> MSLESMLSHPPIPIADMAEHTERLKANDSLKLSQEYESIDPGQQFTWEHSNLEVNKPKNRYANVIAYDHSRVILQPIEGIMGSDYINANYVDGYRRQNAYIATQGPLPETFGDFWRMVWEQRSATIVMMTRLEEKSRIKCDQYWPNRGTETYGFIQVTLLDTIELATFCVRTFSLHKNGSSEKREVRQFQFTAWPDHGVPEYPTPFLAFLRRVKTCNPPDAGPIVVHCSAGVGRTGCFIVIDAMLERIKPEKTVDVYGHVTLMRSQRNYMVQTEDQYSFIHEALLEAVGCGNTEVPARSLYAYIQKLAQVEPGEHVTGMELEFKRLANSKAHTSRFISANLPCNKFKNRLVNIMPYESTRVCLQPIRGVEGSDYINASFIDGYRQQKAYIATQGPLAETTEDFWRMLWENNSTIVVMLTKLREMGREKCHQYWPAE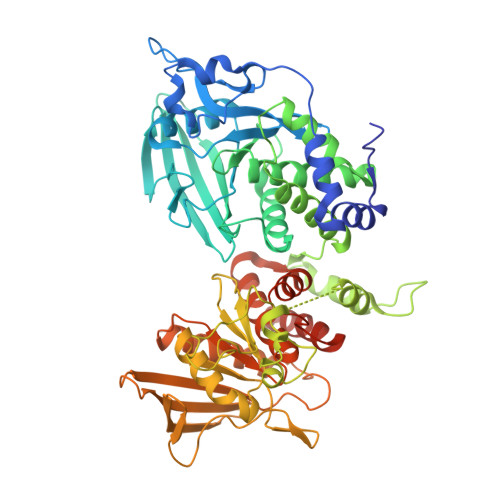RSARYQYFVVDPMAEYNMPQYILREFKVTDARDGQSRTVRQFQFTDWPEQGVPKSGEGFIDFIGQVHKTKEQFGQDGPISVHCSAGVGRTGVFITLSIVLERMRYEGVVDIFQTVKMLRTQRPAMVQTEDEYQFCYQAALEYLGSFDHYATEGHHHHHH>MTTGLSTAGAQDIGRSSVRPYLEECTRRFQEMFDRHVVTRPTKVELTDAELREVIDDCNAAVAPLGKTVSDERWISYVGVVLWSQSPRHIKDMEAFKAVCVLNCVTFVWDDMDPALHDFGLFLPQLRKICEKYYGPEDAEVAYEAARAFVTSDHMFRDSPIKAALCTTSPEQYFRFRVTDIGVDFWMKMSYPIYRHPEFTEHAKTSLAARMTTRGLTIVNDFYSYDREVSLGQITNCFRLCDVSD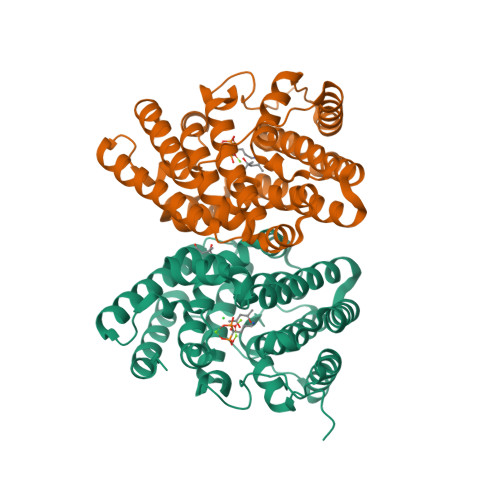ETAFKEFFQARLDDMIEDIECIKAFDQLTQDVFLDLIYGNFVFTTSNKRYKTAVNDVNSRIQAAALEHHHHHH[2x]>MGHHHHHHHHHHSSGHIEGRHMMATNLRGVMAALLTPFDQQQALDKASLRRLVQFNIQQGIDGLYVGGSTGEAFVQSLSERAQVLEIVAEEAKGKIKLIAHVGCVSTAESQQLAASAKRHGFDAVSAVTPFYYPFSLEEHCDH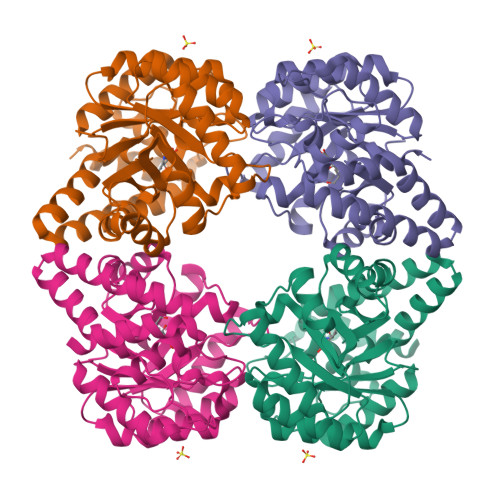YRAIIDSADGLPMVVYNIPALSGVKLTLGQIYTLVTLPGVGALKQTSGDLYQMEQIRREHPDLVLYNGYDEIFASGLLAGADGGIGSTYNIMGWRYQGIVKALKEGDIQTAQKLQTECNKVIDLLIKTGIFRGLKTVLHYMDVISVPLCRKPFGPVDEKCLPELKALAQQLMQERG[4x]> GS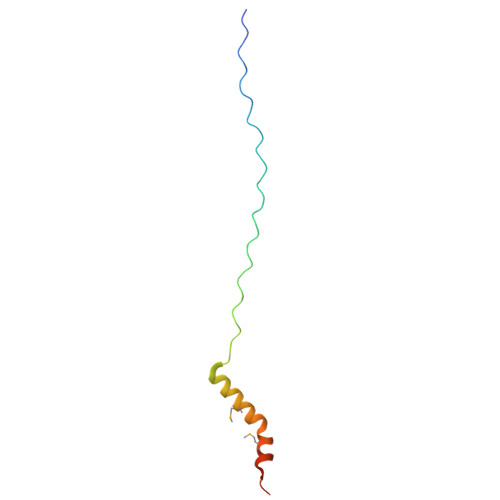GPPGPPGPPGPPGARGEPGNIGFPGPPGPPGPPGRAPTDQHIKQVCMRVIQEHFAEMAASLKRPDSGAT> MGTGKKEKSRRIREGDTKDGNLRVKGENFYRDSKRVKFLNMYTSGKEIRNKKGNLIRAASFQDSTIPDARVQPDRRWFGNTRVISQDALQHFRSALGETQKDTYQVLLRRNKLPMSLLEEKDADESPKARILDTESYADAFGPKAQRKRPRLAASNLEDLVKATNEDITKYEEKQVLDATLGLMGNQEDKENGWTSAAKE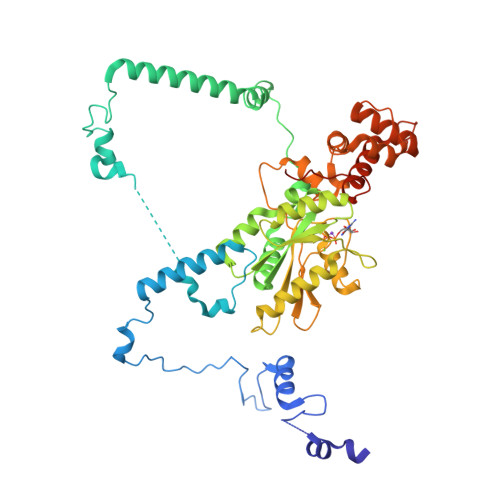AIFSKGQSKRIWNELYKVIDSSDVVIHVLDARDPLGTRCKSVEEYMKKETPHKHLIYVLNKCDLVPTWVAAAWVKHLSKERPTLAFHASITNSFGKGSLIQLLRQFSQLHTDRKQISVGFIGYPNTGKSSIINTLRKKKVCQVAPIPGETKVWQYITLMKRIFLIDCPGIVPPSSKDSEEDILFRGVVRVEHVTHPEQYIPGVLKRCQVKHLERTYEISGWKDATEFIEILARKQGRLLKGGEPDESGVSKQILNDFNRGKIPWFVLPPEKEGEEKPKKKEVEKTA>[60x]MGAIVVTGIPGVGKTTVMQKAAEGSPLPRVPLEGVMYGVAKRMGLVKDIDEMRRLSPDVQKEVQKKAAERIAALGDVILDTHCTIKTPKGYLPGLPRWVLEKLRPSV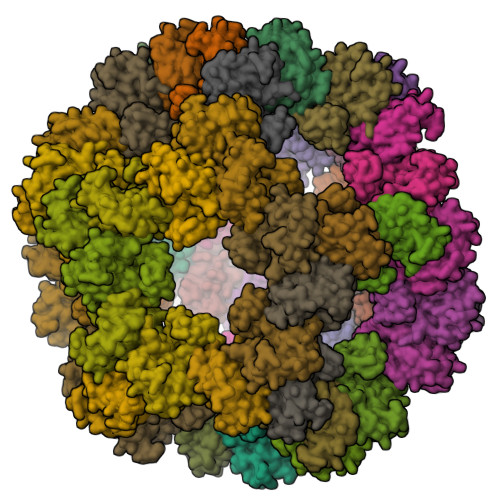ILLVEADPKEIYGRRLKDETRNRDPDSEEEIAEHQMMNRAAAMAYASLSGATVKIVFNHDNRLDDAVRDAAPVLGNLEHHHHHH>[2x]MMTNLETRLSGADPVFARELHAQLVQALGDVKRRLLRGGTQQQYQQWQQEADAIEAGLNIIEKIKGE;>MNVQLKKQLAELA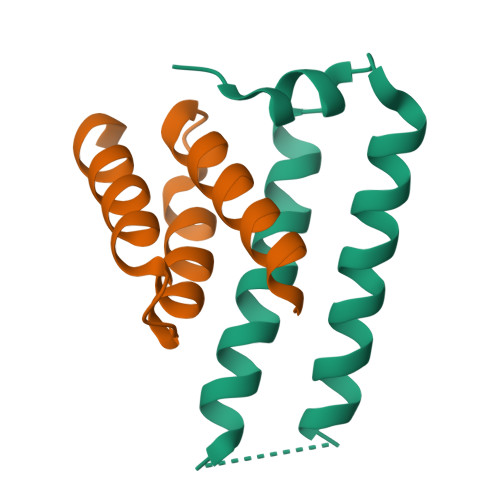LAGTGHHCHQEAASIADWLAQEECMAECVTLIRLSSLMNQGDYQRALL[2x]>GPEPDMISVFIGTWNMGSVPPPKNVTSWFTSKGLGKTLDEVTVTIPHDIYVFGTQENSVGDREWLDLLRGGLKELTDLDYRPIAMQSLWNIKVAVLVKPEHENRISHVSTSSVKTGIANTLGNKGAVGVSFMFNGTSFGFVNCHLTSGNEKTARRNQNYLDILRLLSLGDRQLNAFDISLRFTHLFWFGDLNYRLDMDIQEILNYISRKEFEPLLRVDQLNLEREKHKVFLRFSEEEISFPPTYRYERGSRDTYAWHKQKPTGVRTNVPSWCDRILWKSYPETHIICNSYGCTDDIVTSDHSPVFGTFEVGVTSQFISKKGLSKTSDQAYIEFESIEAIVKTASRTKFFIEFYSTCLEEYKKSFENDAQSSDNINFLKVQWSSRQLPTLKPILADIEYLQDQHLLLTVKSMDGYESYGECVVALKSMIGSTAQQFLTFLSHRGEETGNIRGSMKVRVPTER[8x]

The two main enzymes responsible for PI(3,4,5)P3 degradation are the tumor suppressor phosphatase and tensin homolog (PTEN), which removes the 3-phosphate (3 P) and the SH2-containing inositol 5-phosphatase (SHIP), which dephosphorylates the 5 P to generate PI(3,4)P2. The SHIP Ptase domain belongs to a family of Mg2+-dependent inositol phosphatases with specificity for 5 P dephosphorylation of inositol rings. Here, we report the crystal structure of SHIP2 containing the 5-Ptase and a C2 domain (Ptase-C2), revealing that the two domains tightly associate via an extensive interface. Importantly, even in the absence of a localization effect, the C2 domain provides activating signals to the Ptase active site, resulting in a significant increase in catalytic turnover.

A construct of human SHIP2 containing residues 420–878 corresponding to the Ptase and a C2 domain (Ptase-C2) was crystallized and diffraction data collected to 1.96 Å. The protein crystallized in the P212121 space group with eight molecules per asymmetric unit (for crystallographic and refinement statistics). Each of the eight molecules (A-H) contains a 5-Ptase and a C2 domain. The overall structure of the Ptase domain in Ptase-C2 is similar to the one previously reported, displaying a central β-sheet sandwich decorated by seven helices (α1-α7) and several loops (L1-L4). Importantly, a loop proximal to the active site, spanning residues 674–684 (L4), was in previous Ptase structures disordered or closed over the active site (hereafter referred to as L4-in conformation), whereas in our structure 6 of the Ptase-C2 monomers (A, B, C, E, F, G) exhibit a conformation where L4 points away from the active site (L4-out). These L4-out conformations are stabilized by interactions of R682 in L4 with one or two aspartic acids (D613/D615) adjacent to helix α5 (hereafter referred to as singly or doubly bound L4-out conformations). In molecule D, R682 is half way between the L4-in and L4-out conformation and in monomer H R682 is disordered. Together, these conformations suggest extensive mobility of L4 with a displacement of the guanidinium group of the R682 side chain by ~20 Å between L4-in and L4-out conformations. The Ptase and C2 domains share an extensive interface of 940 Å2, resulting in stabilization of the Ptase. The interface is constituted largely of hydrophobic interactions, with A592, F593, L597, Y697 and P698 in the Ptase and Y770, H820, L822, E836, V838 and A840 in the C2 domain forming a hydrophobic core.>PFTYSIEATRNLATTERCIQDIRNAPVRNRSTQFQLAQQNMLAYTFGEVIPGFASAGINGMDYRDVIGRPVENAVTEGTHFFRDDFRVDSNAKAKVAGDIFEIVSSAVMWNCAARWNSLMVGEGWRSQPRYSRPTLSPSPRRQVAVLNLPRSFDWVSLLVPESQEVIEEFRAGLRKDGLGLPTSTPDLAVVVLPEEFQNDEMWREEIAGLTRPNQILLSGAYQRLQGRVQPGEISLAVAFKRSLRSDRLYQPLYEANVMQLLLEGKLGAPKVEFEVHTLAPEGTNAFVTYEAASLYGLAEGRSAVHRAIRELYVPPTAADLARRFFAFLNERMELVNG[8x]

SgrAI is a type IIF restriction endonuclease that cuts an unusually long recognition sequence and exhibits allosteric self-modulation of cleavage activity and sequence specificity. Previous studies have shown that DNA bound dimers of SgrAI oligomerize into an activated form with higher DNA cleavage rates, although previously determined crystal structures of SgrAI bound to DNA show only the DNA bound dimer. Type II restriction endonucleases typically bind and recognize palindromic sequences as dimers, but the unusual biochemical properties exhibited by SgrAI suggest the formation of a higher order oligomer, containing altered enzymatic properties. A mechanism involving domain swapping is proposed to explain the unusual allosteric properties of SgrAI via association of the domain swapped tetramer of SgrAI bound to DNA into higher order oligomers.

A new crystal structure of the type II restriction endonuclease SgrAI bound to DNA and Ca2+ is now presented, which shows the close association of two DNA bound SgrAI dimers. The new structure of SgrAI described here shows a tetramer that is unlike the NgoMIV and Cfr10I structures, with the tetrameric interface of SgrAI at the DNA binding face of the dimer (i.e. head-to-head) stabilized by the swapping of the amino-terminal 24 residues of each subunit (space filling spheres). The domain swapping, along with other contacts between the two dimers, create a tetramer of SgrAI bound to two DNA duplexes. The crystallographic asymmetric unit contains two such tetramers. Residues 25–30 of each subunit comprise a linker, or hinge loop as it is referred in domain swapped structures, in the domain swapping, as these residues take on a different conformation in the swapped structures than in the previously described unswapped structures. The crystals were grown in a solution containing 50 mM CaCl2, and two Ca2+ are bound in each active site at positions found previously. The contacts to the recognition sequence, CACCGGTG, by SgrAI are identical to those described previously. In both tetramers, composed of A, B, G, and H in tetramer 1 and E, F, C, and D in tetramer 2, the hinge loops are better ordered in one swapped pair than the other. The symmetry within each tetramer shows a small deviation from perfect 222 symmetry, where a total of three 2-fold axes occur orthogonal to one another. Analysis of the active sites of all SgrAI structures solved to date (Dunten et al. 2008 and current work) shows very similar placement of all groups including the DNA in the various crystal structures, indicating that only a single conformation of the enzyme has been determined, which we have argued to be the low activity conformation.>MKQTLLLVEDDKNLADGLLVSLEQAGYECLHVERIADVEPQWKKADLVILDRQLPDGDSVQHLPEWKKIKDVPVILLTALVTVKDKVAGLDSGANDYLTKPFAEAELFARIRAQLRAPDSADQANADKVMTKDLEIDRATREVIFKGDLITLTRTEFDLLLFLASNLGRVFTRDELLDHVWGYNHFPTTRTVDTHVLQLRQKLPGLEIETLRGVGYKMKA[8x]

The response regulator VbrR from Vibrio parahaemolyticus, a member of the OmpR/PhoB family, regulates virulence and antibiotic resistance genes. VbrR is a member of the OmpR/PhoB family and contains an N-terminal receiver domain (RD) and a C-terminal DNA-binding domain (DBD), connected by a flexible linker, and can directly bind with the promoter region of exsC to mediate its downregulation. The VbrK/VbrR TCS is activated by host-derived nitrite during infection, which leads to the downregulation of Type-3 secretion system-1 (T3SS1) via repression of its positive regulator exsC for maximal virulence. In the cell or solution, VbrR proteins exist mainly as inhibitory dimers formed through the DBD, and phosphorylation of RDs allows the formation of RD dimers, which in turn changes the conformation of the DBD from an inhibitory state to an active state.

To gain insights into the DNA binding mode of VbrR, we cocrystallized the monomeric VbrR and DNA fragments of various lengths within the 30 bp fragment, with either blunting ends or overhangs of one or two bases. Crystals of VbrR in complex with a blunt-ended 26 bp DNA fragment were obtained, and the resulting structure of the VbrR-DNA complex was determined to 4.6 Å resolution to allow for the denotation of the secondary structure elements of the RD and DBD domains. Eight molecules, corresponding to four VbrR dimers and two DNA fragments, were modelled in the asymmetric unit. Two dimers (complex-1 and complex-3) bind with DNA fragments in the forward direction, while the other two (complex-2 and complex-4) bind with DNA fragments in the reverse direction, which may be due to crystal packing. We focused on complex-1, which represents the active conformation of VbrR dimer binding with exsC promoter DNA, to analyze structural details. In the VbrR-DNA structure, each VbrR protomer contains one RD and one DBD, connected by a disordered linker. The two RDs form a symmetric head-to-head dimer using the α 4-β 5-α 5 interface, and the two DBDs form a head-to-tail dimer and bind with DNA half-sites S1 (TTCTAAT) and S2 (TTCATCG), respectively. In protomer A, the interaction surface involves α2-α4 from the RD domain and β7-β8 loop, α6, and α7-α8 loop from the DBD domain, whereas it involves α1’, α1’-β2’ loop, and α2’ from the RD domain and α6’, α7’, α7’-α8’ loop from the DBD domain in protomer B. Each DBD places its recognition helix-α8/α8’ into the DNA major groove, where it recognizes 7 bp of promoter DNA, and the C-terminus of α6/α6’ also involves DNA binding. In addition, the β-hairpin connecting β9-β10/β9’-β10’ dips into the DNA minor groove.>[4x]MDKELGKTLRRLRQGKQVSISSLADEHLSKSQISRFERGESEISCSRLLNLLDKLNITIDEFVSTHSKTHTHFFTLLSRVRKYYAEKNVAKLLKLLEDYAHKDYESTMIKAILSSIEPTVEPSEEEVTRLTDYLFSVEQWGYYEIILLGNCSRFINYNTLFLLTKEMVTSFAYSEQNKTNKTL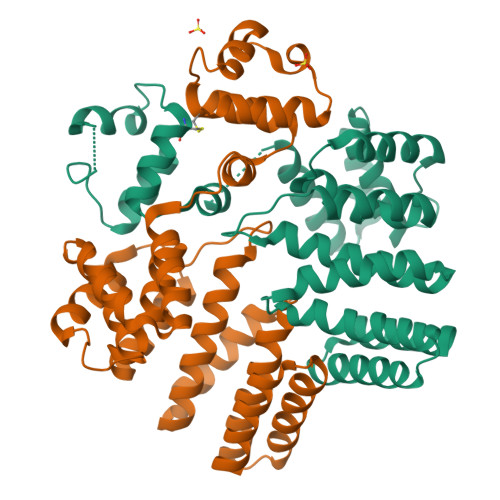VTQLSINCLIISIDYSYFDHSHYLIEKIEFLLRDELNFYEKTVFLYVHGYYKLKQGQVSGKDDMRQALQIFKYLGEDALYYSYKEHYRKEVLGDEEDEEEG N~2~-{2-chloro-4-[(4-methylpiperazin-1-yl)carbonyl]phenyl}-N~2~,N~8~-dimethyl-4,5-dihydrothieno[3,2-d][1]benzoxepine-2,8-dicarboxamide | C28 H29 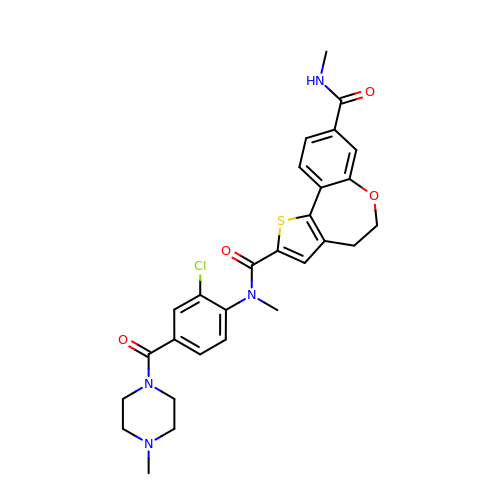Cl N4 O4 S | TVUWQOATJJJPPP-UHFFFAOYSA-N The C-protein C.Esp1396I is a member of a large class of helix-turn-helix proteins that act as transcriptional regulators of gene expression in both prokaryotic and eukaryotic systems. C.Esp1396I finely regulates a bacterial restriction-modification system, providing a delay in endonuclease expression via a concentration-dependent ‘on’ and ‘off’ switch. The C-protein–DNA operator complex consists of two ‘controller’ C-protein dimers (chains A and B, chains C and D) bound to a 35 bp DNA operator sequence (chains E and F). The dsDNA is distorted in the complex, due to binding of protein dimers to each operator site, resulting in minor groove compression (leading to a 50° bend at each binding site) and large major groove expansion at the DNA sequence centre.

To investigate the distribution of specific damage throughout the C.Esp1396I protein–DNA structure with respect to increasing radiation dose, eight successive datasets on the same C.Esp1396I crystal were collected, each exposing the same 100° wedge of the crystal to X-ray radiation. For the later datasets (2 to 8), molecular replacement was performed with PHASER using the refined first dataset final model as the search model. The later datasets were refined only using isotropic B-factor refinement in phenix.refine and were similarly refined to 2.8 Å. For example, by observing the step increases in damage frequency with increasing dose for each residue type, there is a clear difference in the peak detection rate between glutamate and aspartate decarboxylation for doses in the range 6.2 MGy to 35.7 MGy. Clear loss of electron density localized around the carboxyl groups, due to decarboxylation, is shown for Asp64 and Glu54, and the rate of carboxyl electron density loss with dose appears marginally greater for Glu54 than for Asp64. Figs. 5(a)–5(f) also show specific damage to Met57, where electron density loss and side chain disorder can be observed localized on the methylthio group over increasing doses.

>GSHMESFLLSKVSFVIKKIRLEKGMTQEDLAYKSNLDRTYISGIERNSRNLTIKSLELIMKGLEVSDVVFFEMLIKEILKHD[4x]> SSPSPLNPGTNVARLAEQAPIHWVSVAQIENS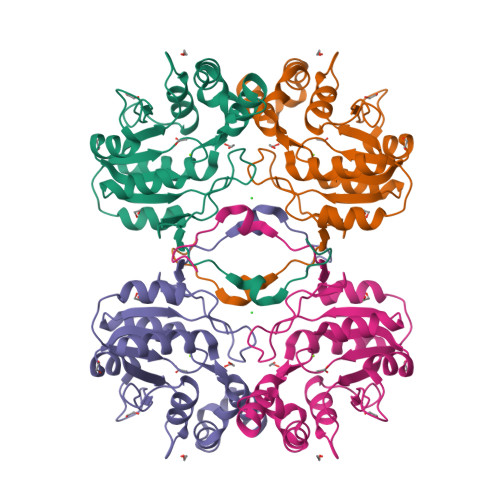LAGRPPMAVGFDIDDTVLFSSPGFWRGKKTFSPESEDYLKNPVFWEKMNNGWDEFSIPKEVARQLIDMHVRRGDAIFFVTGRSPTKTETVSKTLADNFHIPATNMNPVIFAGDKPGQNTKSQWLQDKNIRIFYGDSDNDITAARDVGARGIRILRASNSTYKPLPQAGAFGEEVIVNSEY>[2x]AEVTQLSNGIVVATEHNPSAHTASVGVVFGSGAANENPYNNGVSNLWKNIFLSKENSAVAAKEGLALSSNISRDFQSYIVSSLPGSTDKSLDFLNQSFIQQKANLLSSSNFEATKKSVLKQVQDFEENDHPNRVLEHLHSTAFQNTPLSLPTRGTLESLENLVVADLESFANNHFLNSNAVVVGTGNIKHEDLVNSIESKNLSLQTGTKPVLKKKAAFLGSEVRLRDDTLPKAWISLAVEGEPVNSPNYFVAKLAAQIFGSYNAFEPASRLQGIKLLDNIQEYQLCDNFNHFSLSYKDSGLWGFSTATRNVTMIDDLIHFTLKQWNRLTISVTDTEVERAKSLLKLQLGQLYESGNPVNDANLLGAEVLIKGSKLSLGEAFKKIDAITVKDVKAWAGKRLWDQDIAIAGTGQIEGLLDYMRIRSDMSMMRW;>[2x]LTVSARDAPTKISTLAVKVHGGSRYATKDGVAHLLNRFNFQNTNTRSALKLVRESELLGGTFKSTLDREYITLKATFLKDDLPYYVNALADVLYKTAFKPHELTESVLPAARYDYAVAEQCPVKSAEDQLYAITFRKGLGNPLLYDGVERVSLQDIKDFADKVYTKENLEVSGENVVEADLKRFVDESLLSTLPAGKSLVSKSEPKFFLGEENRVRFIGDSVAAIGIPVNKASLAQYEVLANYLTSALSELSGLISSAKLDKFTDGGLFTLFVRDQDSAVVSSNIKKIVADLKKGKDLSPAINYTKLKNAVQNESVSSPIELNFDAVKDFKLGKFNYVAVGDVSNLPYLDEL;>MAFRKSNVYLSLVNSYIIDSPQPSSINYWWNMGSLLGLCLVIQIVTGIFMAMHYSSNIELAFSSVEHIMRDVHNGYILRYLHANGASFFFMVMFMHMAKGLYYGSYRSPRVTLWNVGVIIFILTIATAFLGYCCVYGQMSHWGATVITNLFSAIPFVGNDIVSWLWGGFSVSNPTIQRFFALHYLVPFIIAAMVIMHLMALHIHGSSNPLGITGNLDRIPMHSYFIFKDLVTVFLFMLILALFVFYSPNTLGHPDNYIPGNPLVTPASIVPEWYLLPFYAILRSIPDKLLGVITMFAAILVLLVLPFTDRSVVRGNTFKVLSKFFFFIFVFNFVLLGQIGACHVEVPYVLMGQIATFIYFAYFLIIVPVISTIENVLFYIGRVNK[2x];>[2x]MTAAEHGLHAPAYAWSHNGPFETFDHASIRRGYQVYREVCAACHSLDRVAWRTLVGVSHTNEEVRNMAEEFEYDDEPDEQGNPKKRPGKLSDYIPGPYPNEQAARAANQGALPPDLSLIVKARHGGCDYIFSLLTGYPDEPPAGVALPPGSNYNPYFPGGSIAMARVLFDDMVEYEDGTPATTSQMAKDVTTFLNWCAEPEHDERKRLGLKTVIILSSLYLLSIWVKKFKWAGIKTRKFVFNPPKPRK;>[2x]KSTYRTPNFDDVLKENNDADKGRSYAYFMVGAMGLLSSAGAKSTVETFISSMTATADVLAMAKVEVNLAAIPLGKNVVVKWQGKPVFIRHRTPHEIQEANSVDMSALKDPQTDADRVKDPQWLIMLGICTHLGCVPIGEAGDFGGWFCPCHGSHYDISGRIRKGPAPLNLEIPAYEFDGDKVIVG;>[2x]MGMLELVGEYWEQLKITVVPVVAAAEDDDNEQHEEKAAEGEEKEEENGDEDEDEDEDEDDDDDDDEDEEEEEEVTDQLEDLREHFKNTEEGKALVHHYEECAERVKIQQQQPGYADLEHKEDCVEEFFHLQHYLDTATAPRLFDKLK;>MPQSFTSIARIGDYILKSPVLSKLCVPVANQFINLAGYKKLGLKFDDLIAEENPIMQTALRRLPEDESYARAYRIIRAHQTELTHHLLPRNEWIKAQEDVPYLLPYILEAEAAAKEKDELDNIEVSK[2x];>[2x]MGPPSGKTYMGWWGHMGGPKQKGITSYAVSPYAQKPLQGIFHNAVFNSFRRFKSQFLYVLIPAGIYWYWWKNGNEYNEFLYSKAGREELERVNV;>[2x]MSFSSLYKTFFKRNAVFVGTIFAGAFVFQTVFDTAITSWYENHNKGKLWKDVKARIAAGDGDDDDE;>MAYTSHLSSKTGLHFGRLSLRSLTAYAPNLMLWGGASMLGLFVFTEGWPKFQDTLYKKIPLLGPTLEDHTPPEDKPN[2x];> MVQRWLYSTNAKDIAVLYFMLAIFSGMAGTAMSLIIRLELAAPGSQYLHGNSQLFNVLVVGHAVLMIFFLVMPALIGGFGNYLLPLMIGATDTAFPRINNIAFWVLPMGLVCLVTSTLVESGAGTGWTVYPPLSSIQAHSGPSVDLAIFALHLTSISSLLGAINFIVTTLNMRTNGMTMHKLPLFVWSIFITAFLLLLSLPVLSAGITMLLLDRNFNTSFFEVSGGGDPILYEHLFWFFGHPEVYILIIPGFGIISHVVSTYSKKPVFGEISMVYAMASIGLLGFLVWSHHMYIVGLDADTRAYFTSATMIIAIPTGIKIFSWLATIHGGSIRLATPMLYAIAFLFLFTMGGLTGVALANASLDVAFHDTYYVVGHFHYVLSMGAIFSLFAGYYYWSPQILGLNYNEKLAQIQFWLIFIGANVIFFPMHFLGINGMPRRIPDYPDAFAGWNYVASIGSFIATLSLFLFIYILYDQLVNGLNNKVNNKSVIYNKAPDFVESNTIFNLNTVKSSSIEFLLTSPPAVHSFNTPAVQS;> DVPTPYACYFQDSATPNQEGILELHDNIMFYLLVILGLVSWMLYTIVMTYSKNPIAYKYIKHGQTIEVIWTIFPAVILLIIAFPSFILLYLCDEVISPAMTIKAIGYQWYWKYEYSDFINDSGETVEFESYVIPDELLEEGQLRLLDTDTSMVVPVDTHIRFVVTAADVIHDFAIPSLGIKVDATPGRLNQVSALIQREGVFYGACSELCGTGHANMPIKIEAVSLPKFLEWLNEQ;> MTHLERSRHQQHPFHMVMPSPWPIVVSFALLSLALSTALTMHGYIGNMNMVYLALFVLLTSSILWFRDIVAEATYLGDHTMAVRKGINLGFLMFVL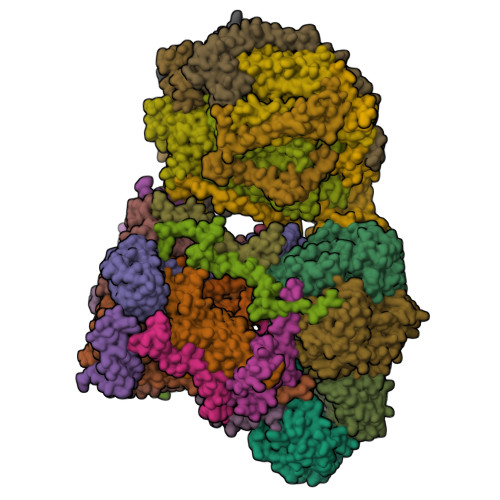SEVLIFAGLFWAYFHSAMSPDVTLGACWPPVGIEAVQPTELPLLNTIILLSSGATVTYSHHALIAGNRNKALSGLLITFWLIVIFVTCQYIEYTNAAFTISDGVYGSVFYAGTGLHFLHMVMLAAMLGVNYWRMRNYHLTAGHHVGYETTIIYTHVLDVIWLFLYVVFYWWGV;> QQKPVVKTAQNLAEVNGPETLIGPGAKEGTVPTDLDQETGLARLELLGKLEGIDVFDTKPLDSSRKGTMKDPIIIESYDDYRYVGCTGSPAGSHTIMWLKPTVNEVARCWECGSVYKLNPVGVPNDDHHH;> VQTKALSKATLTDLPERWENMPNLEQKEIADNLTERQKLPWKTLNNEEIKAAWYISYGEWGPRRPVHGKGDVAFITKGVFLGLGISFGLFGLVRLLANPETPKTMNREWQLKSDEYLKSKNANPWGGYSQVQSK;> SDAHDEETFEEFTARYEKEFDEAYDLFEVQRVLNNCFSYDLVPAPAVIEKALRAARRVNDLPTAIRVFEALKYKVENEDQYKAYLDELKDVRQELGVPLKEELFPSSS;> ANKVIQLQKIFQSSTKPLWWRHPRSALYLYPFYAIFAVAVVTPLLYIPNAIRGIKAKKA;> VHFKDGVYENIPFKVKGRKTPYALSHFGFFAIGFAVPFVACYVQLKKSGAF;> TIAPITGTIKRRVIMDIVLGFSLGGVMASYWWWGFHMDKINKREKFYAELAERKK;> ADQENSPLHTVGFDARFPQQNQTKHCWQSYVDYHKCVNMKGEDFAPCKVFWKTYNALCPLDWIEKWDDQREKGIFAGDINSD;> ASSLPPNALKPAFGPPDKVAAQKFKESLMATEKHAKDTSNMWVKISVWVALPAIALTAVNTYFVEKEHAEHREHLKHVPDSEWPRDYEFMNIRSKPFFWGDGDKTLFWNPVVNRHIEHDDGARGSHHHHHH;> MFFSQVLRSSARAAPIKRYTGGRIGESWVITEGRRLIPEIFQWSAVLSVCLGWPGAVYFFSKARKA;> MKILTQDEIEAHRSHTLKGGIEGALAGFAISAIIFKVLPRRYPKFKPSTLTWSIKTALWITPPTVLTAICAEEASNNFDATMYGSGSSSEDALDEHRRWKSLSTKDKFVEGLSNNKYKIITGAWAASLYGSWVIVNKDPIMTKAQKIVQARMYAQFITVGLLLASVGLSMYENKLHPNKQKVNEMRRWENALRVAEEEERLEKEGRRTGYVSNEERINSKIFKS>GSHNASLTEIEHLVQSVCKSYRETCQLRLEDLLRQRSNIFSREEVTGYQRKSMWEMWERCAHHLTEAIQYVVEFAKRLSGFMELCQNDQIVLLKAGAMEVVLVRMCRAYNADNRTVFFEGKYGGMELFRALGCSELISSIFDFSHSLSALHFSEDEIALYTALVLINAHRPGLQEKRKVEQLQYNL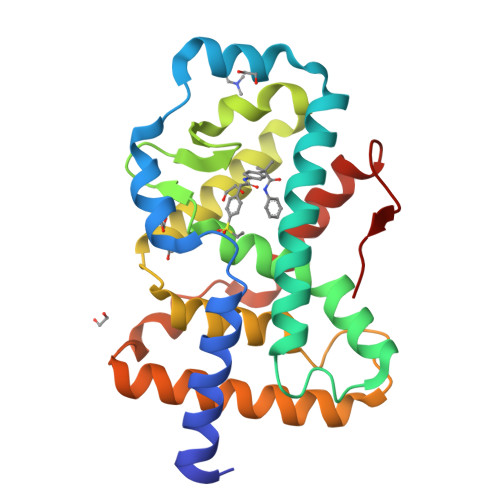ELAFHHHLCKTHRQSILAKLPPKGKLRSLCSQHVERLQIFQHLHPIVV[2x]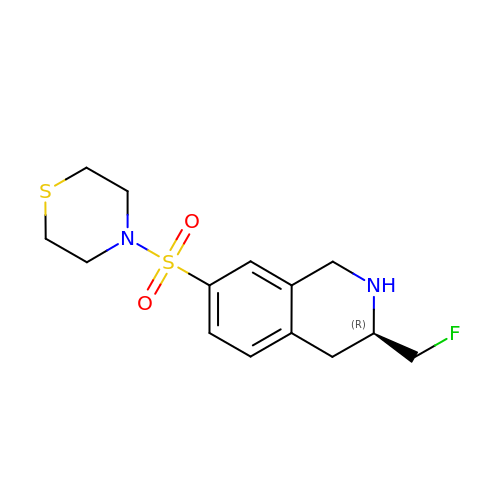(3R)-3-(FLUOROMETHYL)-7-(THIOMORPHOLIN-4-YLSULFONYL)-1,2,3,4-TETRAHYDROISOQUINOLINE | C14 H19 F N2 O2 S2 | SBUKSNPHYWXCDG-CYBMUJFWSA-N> GPGSEFELPLPEGWEEARDFDGKVYY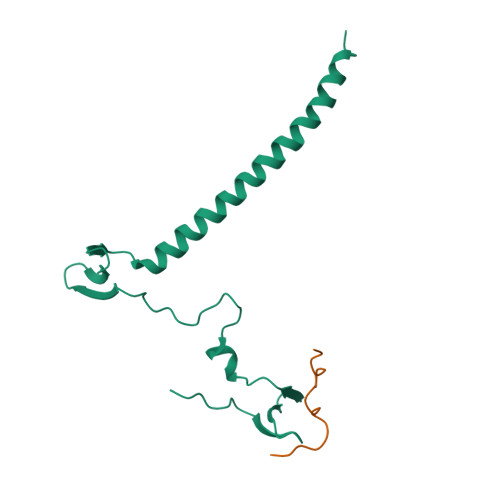IDHRNRTTSWIDPRDRYTKPLTFADCISDELPLGWEEAYDPQVGDYFIDHNTKTTQIEDPRVQWRREQEHMLKDYLVVAQEALSAQKEIYQVKQQRLELAQQEYQQLH;> DRPPPYVAPPSYEGPHRTLGTKRGP> GSEPVKYGELVVLGYNGALPNGDRGRRKSRFALYKRPKANGVKPSTVHMISTPQASKAISCKGQHSISYTLSRNQTVVVEYTHDKDTDMFQVGRSTESPIDFVVTDTISGSQNTDEAQITQSTISRFACRIVCDRNEPYTARIFAAGFDSSKNIFLGEKAAKWKNPDGHMDGLTTNGVLVMHPRGGFTEESQPGVWREISVCGDVYTLRETRSAQQRGKMVESETNVLQDGSLIDLCGATLLWRTADGLFHTPTQKH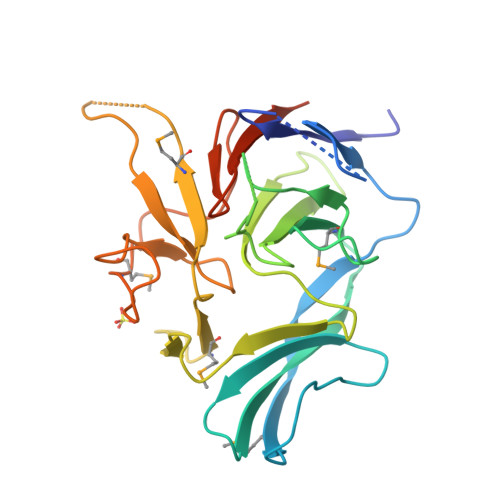IEALRQ>CGCGUCACACCGGUGAAG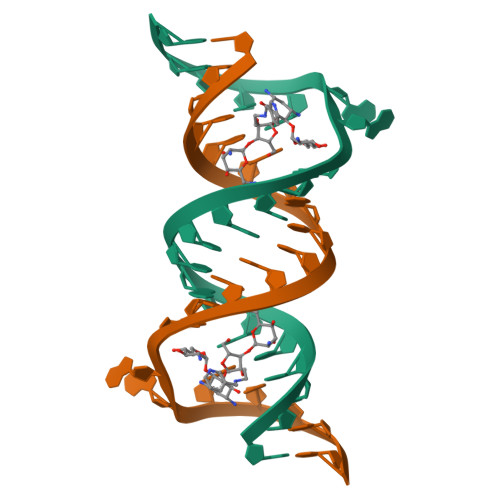UCGC[2x]> GNVVIEVDMANGWRGNASGSTSHSGITYSADGVTFAALGDGVGAVFDIARPTTLEDAVIAMVVNVSAEFKASEANLQIFAQLKEDWSKGEWDCLAGSSELTADTDLTLTCTIDEDDDK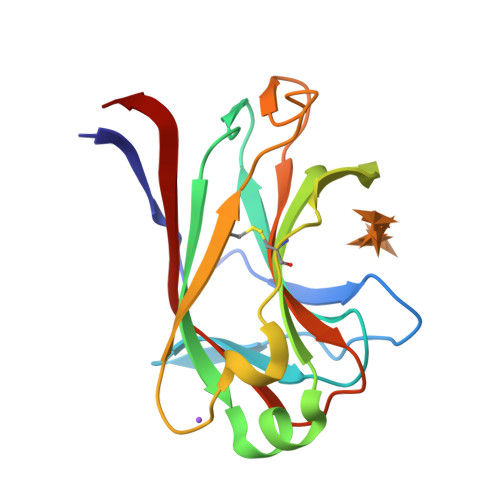FNQTARDVQVGIQAKGTPAGTITIKSVTITLAQEA>MGESKRTEKTRVLVVGATGYIGKRIVRACLAEGHETYVLQRPEIGLEIEKVQLFLSFKKLGARIVEGSFSDHQSLVSAVKLVDVVVSAMSGVHFRSHNILVQLKLVEAIKEAGNV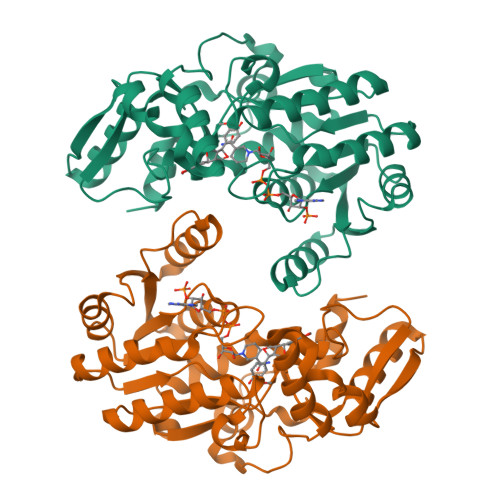KRFLPSEFGMDPPRMGHALPPGRETFDQKMEVRQAIEAAGIPYTYVVGACFAAYFAGNLSQMVTLLPPKEKVNIYGDGNVKVVFADEDDIAKYTAKTLNDPRTLNKTVNIRPPDNVLTQLELVQIWEKLTGKELEKTNIAAQDFLANIEQMEIPHQAGIGHFYHIFYEGCLTDHEVGEDEEASSLYPDVKYKRMDDYLRMFL[4x]> MSAFTPASEVLLRHSDDFEQSRILFAGDLQDDLPARLDTAASRAHTQQFHHWQVLSRQMGDNARFSLVATADDVADCDTLIYYWPKNKPEAQFQLMNLLSLLPVGTDIFVV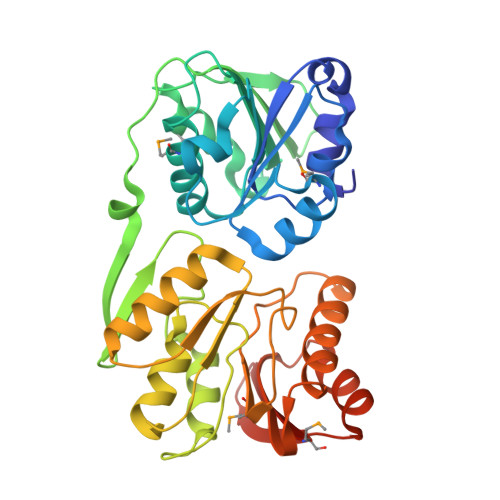GENRSGVRSAEQMLADYAPLNKVDSARRCGLYFGRLEKQPVFDAEKFWGEYSVDGLTVKTLPGVFSRDGLDVGSQLLLSTLTPHTKGKVLDVGCGAGVLSVAFARHSPKIRLTLCDVSAPAVEASRATLAANGVEGEVFASNVFSEVKGRFDMIISNPPFHDGMQTSLDAAQTLIRGAVRHLNSGGELRIVANAFLPYPDVLDETFGFHEVIAQTGRFKVYRAIMTRQAKKG> GSHMGEVKSVKVDNWGVFFLQKLQNFFNKTDYCDL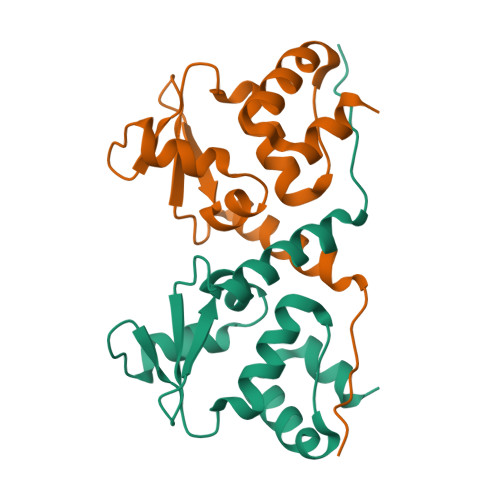TLQFRDNSQLKVHRLVLSACTDYFNVLEQTCEIVDDALIMPNEFQADVVVPIVNFMYTGTLEFELKMYGKLLRTAKEMNMTVLLKLLEAHRRTMENVNRQQRP5-(5-(6-CHLORO-4-(4,5-DIHYDRO-2-OXAZOLYL)PHENOXY)PENTYL)-3-METHYL 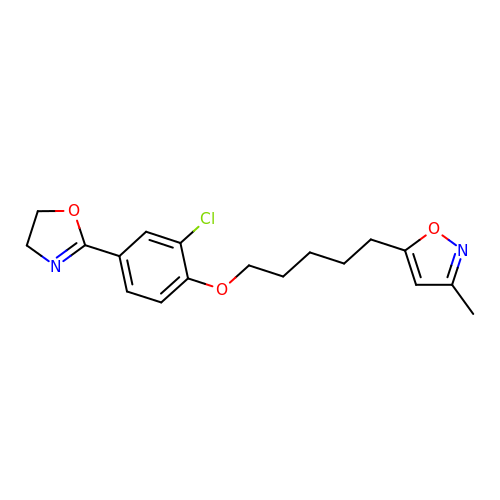ISOXAZOLE | C18 H21 Cl N2 O3 | FCSKOFQQCWLGMV-UHFFFAOYSA-N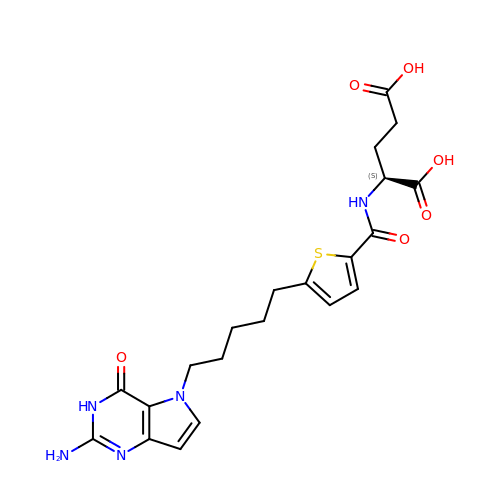N-{5-[5-(2-amino-4-oxo-3,4-dihydro-5H-pyrrolo[3,2-d]pyrimidin-5-yl)pentyl]thiophene-2-carbonyl}-L-glutamic acid | C21 H25 N5 O6 S | RQAHNHUMMCUWMX-AWEZNQCLSA-N>SNAMDSSASVVFMRFAPPGEETALPPRRATPGSVAYDLFPSEEMDIEPMGLAKISTGYGIDKFPDGCYGQIVSRSGMTWKNNTSVPTGTIDVDYRGELKVILRNHSAEKSVPIRKGTSIAQLIFLRY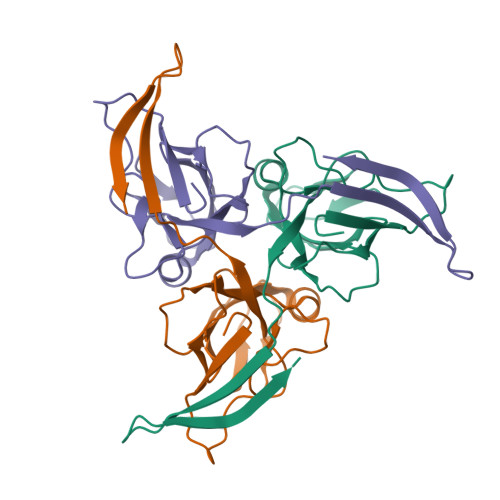CDVEEEQIVYINETTGERTIIDSSSKKDNKNQARSVRGTGGFGSTDN[6x]>[2x]PGSEFELGNKGNNILNSNESRLNVNENNILREKFENYARIVFQFNNS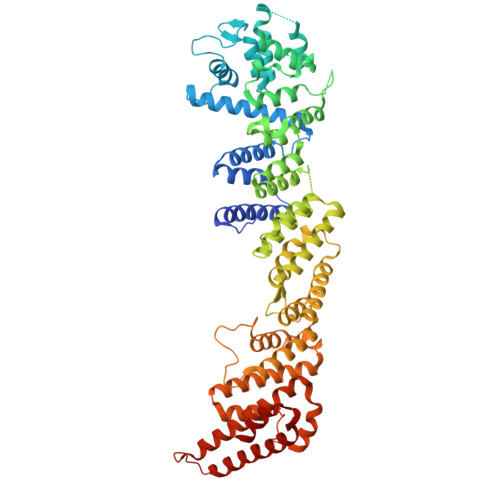RQANGNFDIANEFISILSSANGTRNAQLLESWKILESMKSKDINIVEVGKQYLEQQFLQYTDNLYKKNMNEGLATNVNKIKSFIDTKLKKADKSWKISNLTVINGVPIWALIFYLLRAGLIKEALQVLVENKANIKKVEQSFLTYFKAYASSKDHGLPVEYSTKLHTEYNQHIKSSLDGDPYRLAVYKLIGRCDLSRKNIPAVTLSIEDWLWMHLMLIKEKDAENDPVYERYSLEDFQNIIISYGPSRFSNYYLQTLLLSGLYGLAIDYTYTFSEMDAVHLAIGLASLKLFKIDSSTRLTKKPKRDIRFANILANYTKSFRYSDPRVAVEYLVLITLNEGPTDVELCHEALRELVLETKEFTVLLGKIGRDGARIPGVIEERQPLLHVRDEKEFLHTITEQAARRADEDGRIYDSILLYQLAEEYDIVITLVNSLLSDTLSASDLDQPLVGPDDNSETNPVLLARRMASIYFDNAGISRQIHVKNKEICMLLLNISSIRELYFNKQWQETLSQMELLDLLPFSDELSARKKAQDFSNLDDNIVKNIPNLLIITLSCISNMIHILNESKYQSSTKGQQIDSLKNVARQCMIYAGMIQYRMPRETYSTLINIDVSL> MWSHPAVRKSSSKTIRSRSIWDDAHAMLEKAKAEGISTVWDRAAEQTPAAKFAELGTTCRNCIMGPCRIANRKDGKMRLGVCGADADVIVARNFGRFIAGGAAGHSDHGRDLIETLEAVAEGKAPGYTIRDVAKLRRIAAELGVADAATRPAHDVAADLVTICYNDFGSRRNALAFLARAPQVRRDLWQRLGMTPRGVDREIAEMMHRTHMGCDNDHTSLLVHAARTALADGWGGSMIGTELSDILFGTPRPRQSTVNLGVLRKDAVNILVHGHNPVVSEMILAATREPAVRQAAQDAGAADINVAGLCCTGNELLMRQGIPMAGNHLMTELAIVTGAADAIVADYQCIMPSLVQIAACYHTRFVTTSPKGRFTGATHVEVHPHNAQERCREIVMLAIDAYTRRDPARVDIPSQPVSIMSGFSNEAILEALGGTPKPLIDAVVAGQIRGFVGIVGCNNPKIRQDSANVTLTRELI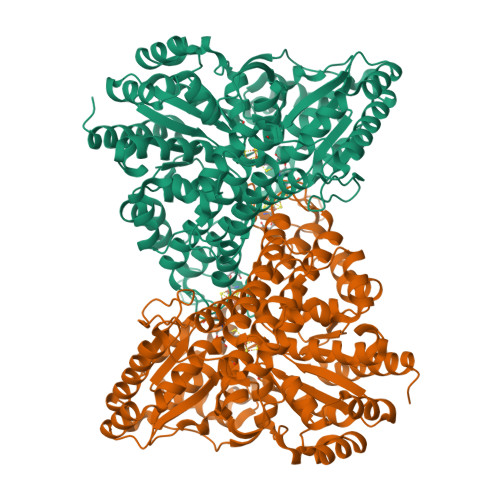RRDIMVLATGCVTTAAGKAGLLVPEAASKAGEGLAAVCRSLGVPPVLHMGSCVDNSRILQLCALLATTLGVDISDLPVGASSPEWYSEKAAAIAMYAVASGIPTHLGLPPNILGSENVTAMALHGLQDVVGAAFMVEPDPVKAADMLEAHIVARRARLGLTS>[4x]GPMASQPNSSAKKKEEKGKNIQVVVRCRPFNLAERKASAHSIVECDPVRKEVSVRTGGLADKSSRKTYTFDMVFGASTKQIDVYRSVVCPILDEVIMGYNCTIFAYGQTGTGKTFTMEGER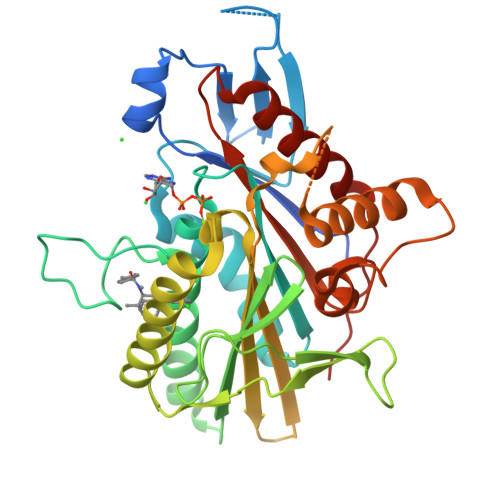SPNEEYTWEEDPLAGIIPRTLHQIFEKLTDNGTEFSVKVSLLEIYNEELFDLLNPSSDVSERLQMFDDPRNKRGVIIKGLEEITVHNKDEVYQILEKGAAKRTTAATLMNAYSSRSHSVFSVTIHMKETTIDGEELVKIGKLNLVDLAGSENIGRSGAVDKRAREAGNINQSLLTLGRVITALVERTPHVPYRESKLTRILQDSLGGRTRTSIIATISPASLNLEETLSTLEYAHRAKNILNKPEVNQK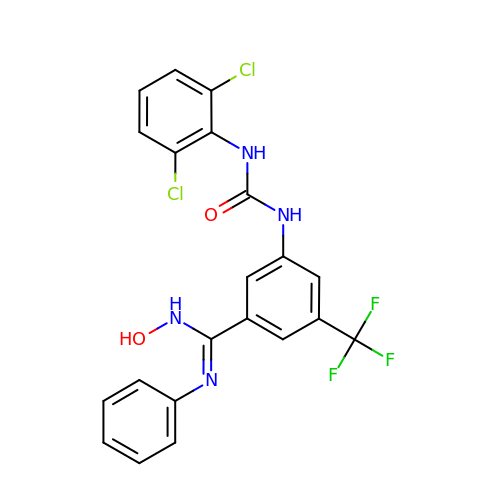3-{[(2,6-dichlorophenyl)carbamoyl]amino}-N-hydroxy-N'-phenyl-5-(trifluoromethyl)benzenecarboximidamide | C21 H15 Cl2 F3 N4 O2 | CPPHCXNOGUJCGB-UHFFFAOYSA-N>[2x]GSTLTYPFHDWSQELSPRYAQLRASDAPVCPVVSEGTGDPLWLVTRYATAVKLLEDSRFSSEAAQASGAPRQEPVELRAPGTRGDAIAMLREAGLRSVLADGLGPRAVRRHQGWIND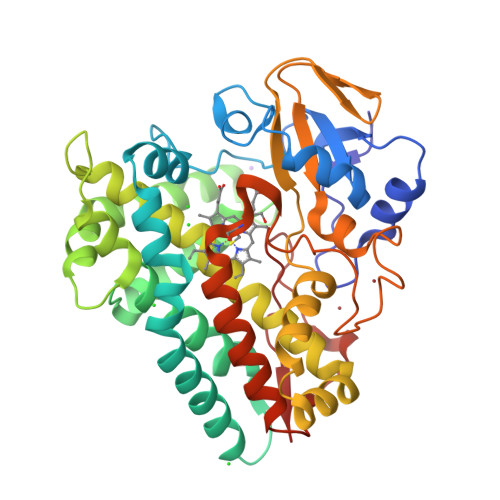LAETLMSELASREGTFDLAADFVEPLSSALVSRTLLGELSADERDLLAHCADTGLRFCGVTHEEQVHAFTQMHEFFLEHARRLAGTPGEHLLKLIAEAPVDQGPLSDEALAEAGSLLVVAGFPTSSGFLCGALLTLLRHPDAVQELHAHPERVPSAVEELLRYTPLSTGSVKRMATEDLEIDGVRIKAGEVVMVSLEAVNHDPDAFEDPDVFRPGREGPMHFGFGRGRHFCPGNRLARCVIEATVRAVARRPGLRLAVAPEEISWHEGLFFRRPRAIPATW>[3x]GLKEHDFNPEEAEETKQVSWKLVTEYAMETKCDDVLLLLGMYLEFQYSFEMCLKCIKKEQPSHYKYHEKHYANAAIFADSKNQKTICQQAVDTVLAKKRVDSLQLTREQMLTNRFNDLLDRMDIMFGSTGSADIEEWMAGVAWLHCLLPKMDSVVYDFLKCMVYNIPKKRYWLFKGPIDSGKTTLAAALLELCGGKALNVNLPLDRLNFELGVAIDQFLVVFEDVKGTGGESRD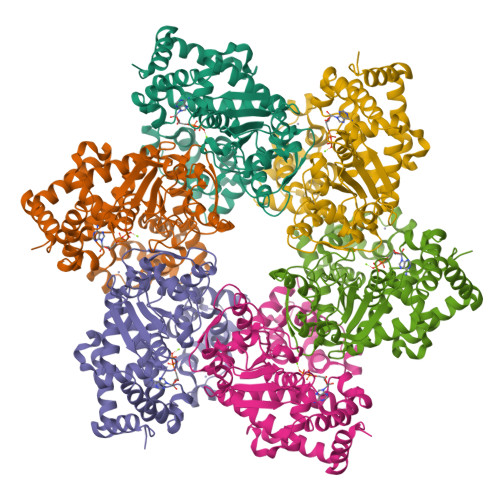LPSGQGINNLDNLRDYLDGSVKVNLEKKHLNKRTQIFPPGIVTMNEYSVPKTLQARFVKQIDFRPKDYLKHCLERSEFLLEKRIIQSGIALLLMLIWYRPVAEFAQSIQSRIVEWKERLDKEFSLSVYQKMKFNVAMGIGVLD>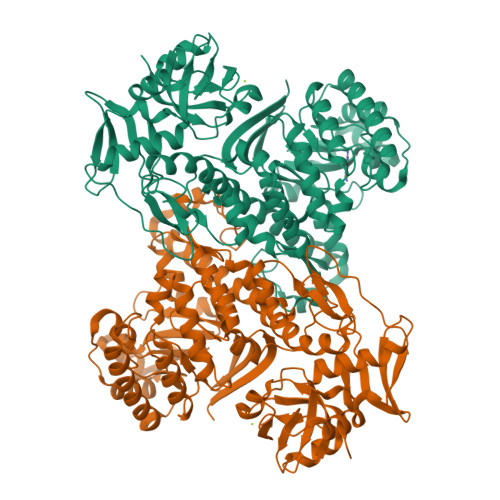[2x]MSRGDKMLKFEIKARDGAGRIGKLEVNGKKIETPAIMPVVNPKQMVVEPKELEKMGFEIIITNSYIIYKDEELRRKALELGIHRMLDYNGIIEVDSGSFQLMKYGSIEVSNREIIEFQHRIGVDIGTFLDIPTPPDAPREQAVKELEITLSRAREAEEIKEIPMNATIQGSTYTDLRRYAARRLSSMNFEIHPIGGVVPLLESYRFRDVVDIVISSKMALRPDRPVHLFGAGHPIVFALAVAMGVDLFDSASYALYAKDDRYMTPEGTKRLDELDYFPCSCPVCSKYTPQELREMPKEERTRLLALHNLWVIKEEIKRVKQAIKEGELWRLVDERARSHPKLYSAYKRLLEHYTFLEEFEPITKKSALFKISNESLRWPVVRRAKERAKSINERFGELVEHPIFGRVSRYLSLTYPFAQSEAEDDFKIEKPTKEDAIKYVMAIAEYQFGEGASRAFDDAKVELSKTGMPRQVKVNGKRLATVRADDGLLTLGIEGAKRLHRVLPYPRMRVVVNKEAEPFARKGKDVFAKFVIFADPGIRPYDEVLVVNENDELLATGQALLSGREMIVFQYGRAVKVRKGVE>[4x]GAMGSEQRASLDSEESESPPQENSCLDPPDRDPNCKPPPVKPHIFTTRSRTRLFGKGDSEEASPLDCPYEEGGLASCPIITVSSVLTIQRPGDGPASVRPSSQDSVSAGEKPPRLYDRRSIFDAVAQSNCQELE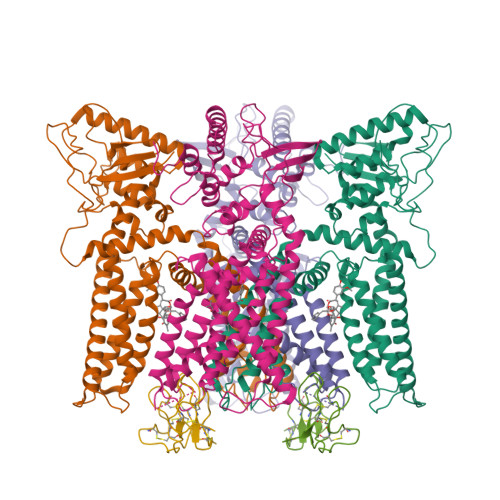SLLPFLQRSKKRLTDSEFKDPETGKTCLLKAMLNLHNGQNDTIALLLDVARKTDSLKQFVNASYTDSYYKGQTALHIAIERRNMTLVTLLVENGADVQAAANGDFFKKTKGRPGFYFGELPLSLAACTNQLAIVKFLLQNSWQPADISARDSVGNTVLHALVEVADNTVDNTKFVTSMYNEILILGAKLHPTLKLEEITNRKGLTPLALAASSGKIGVLAYILQREIHEPECRHLSRKFTEWAYGPVHSSLYDLSCIDTCEKNSVLEVIAYSSSETPNRHDMLLVEPLNRLLQDKWDRFVKRIFYFNFFVYCLYMIIFTAAAYYRPVEGLPPYKLKNTVGDYFRVTGEILSVSGGVYFFFRGIQYFLQRRPSLKSLFVDSYSEILFFVQSLFMLVSVVLYFSQRKEYVASMVFSLAMGWTNMLYYTRGFQQMGIYAVMIEKMILRDLCRFMFVYLVFLFGFSTAVVTLIEDGKNNSLPMESTPHKCRGSACKPGNSYNSLYSTCLELFKFTIGMGDLEFTENYDFKAVFIILLLAYVILTYILLLNMLIALMGETVNKIAQESKNIWKLQRAITILDTEKSFLKCMRKAFRSGKLLQVGFTPDGKDDYRWCFRVDEVNWTTWNTNVGIINEDPGNCEGVKRTLSFSLRSGRVSGRNWKNFALVPLLRDASTRDRHATQQEEVQLKHYTGSLKPEDAEVFKDSMVPGEK;>MDCAKEGEVCSWGKKCCDLDNFYCPMEFIPHCKKYKPYVPVTTNCAKEGEVCGWGSKCCHGLDCPLAFIPYCEKYR[2x]(2~{R},3~{R},4~{S},5~{R})-2-[8-[3-[[(2~{R},3~{S},4~{R},5~{R})-5-(6-aminopurin-9-yl)-3,4-bis(oxidanyl)oxolan-2-yl]methoxy]prop-1-ynyl]-6-azanyl-purin-9-yl]-5-(hydroxymethyl)oxolane-3,4-diol | C23 H26 N10 O8 | 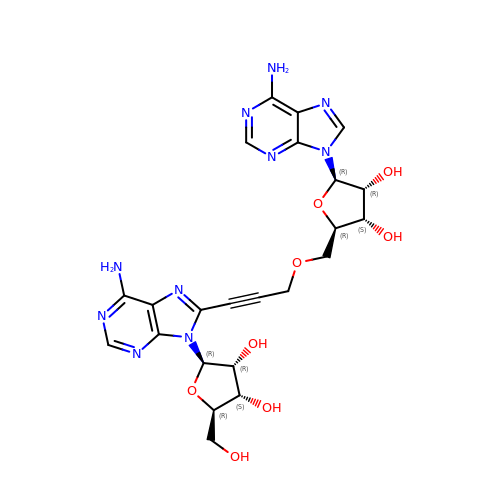DDNDMZZNOIOKKS-MKWZPUSRSA-N> CA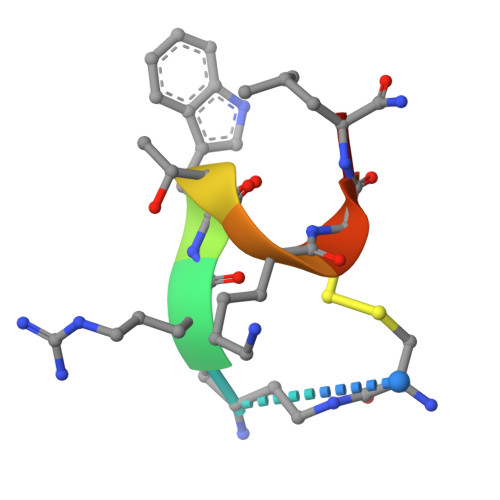RWTKCLX2-(2,2-diphosphonoethyl)-1-propylpyridin-1-ium | C10 H18 N O6 P2 | 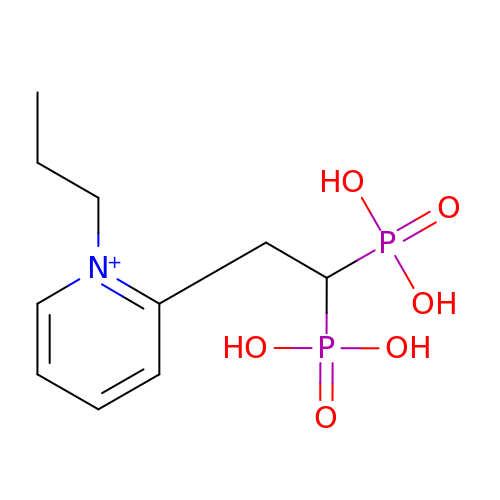KNULKELAVSFYBS-UHFFFAOYSA-O> SFTMTWLPLNPIPLKDRVSMIFLQYGQIDVIDGAFVLIDKTGIRTHIPVGSVACIMLEPGTRVSHAAVRLAAQVGTLLVWVGEAGVRVYASGQPGGARSDKLLYQAKLALDEDLRLKVVRKMFELRFGEPAPARRSVEQLRGIEGSRVRA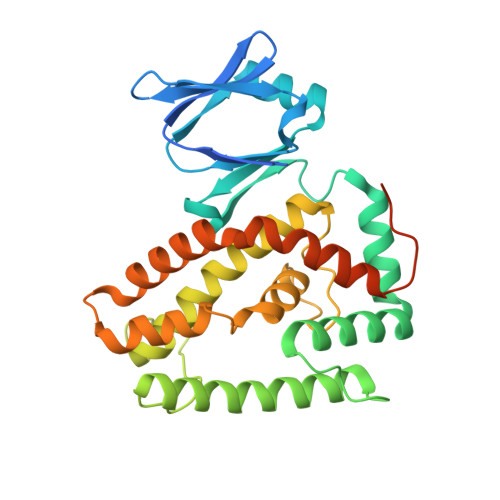TYALLAKQYGVTWNGRRYDPKDWEKGDTINQCISAATSCLYGVTEAAILAAGYAPAIGFVHTGKPLSFVYDIADIIKFDTVVPKAFEIARRNPGEPDREVRLACRDIFRSSKTLAKLIPLIEDVLAAGEIQPPAPPEDAQPVAIPLPVSLGDAGHRSS> MIEIKDKQLTGLRFIDLFAGLGGFRLALESCGAECVYSNEWDKYAQEVYEMNFGEKPEGDITQVNEKTIPDHDILCAGFPCQAFSISGKQKGFEDSRGTLFFDIARIVREKKPKVVFMENVKNFASHDNGNTLEVVKNTM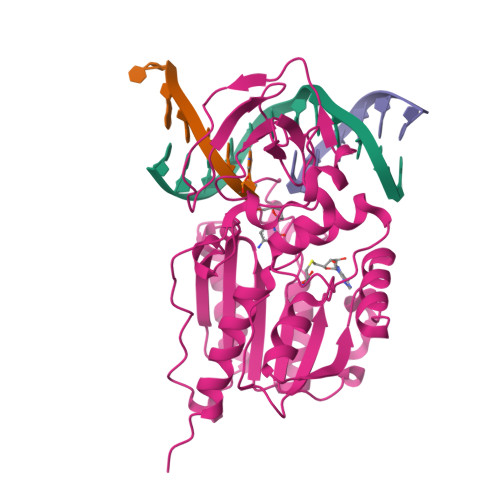NELDYSFHAKVLNALDYGIPQKREAIYMICFRNDLNIQNFQFPKPFELNTFVKDLLLPDSEVEHLVIDRKDLVMTNQEIEQTTPKTVRLGIVGKGGQGERIYSTRGIAITLSAYGGGIFAKTGGYLVNGKTRKLHPRECARVMGYPDSYKVHPSTSQAYKQFGNSVVINVLQYIAYNIGSSLNFKPY> MDPQGDAAQKTDTSHHDQDHPTFNKITPNLAEFAFSLYRQLAHQSNSTNILFSPVSIAAAFAMLSLGAKGDTHDEILEGLNFNLTEIPEAQIHEGFQELLHTLNQPDSQLQLTTGNGLFLSEGLKLVDKFLEDVKKLYHSEAFTVNFGDTEEAKKQINDYVEKGTQGKIVDLVKELDRDTVFALVNYIFFKGKWERPFEVKDTEEEDFHVDQVTTVKVPMMKRLGMFNIQHSKKLSSWVLLMKYLGNATAIFFLPDEGKLQHLENELTHDIITKFLENEDRRSASLHLPKLSITGTYDLKSVLGQLGITKVFSNGADLSGVTEEAPLKLSKAVHKAVLTIDEKGTEAAGAMFLEAIPM;> SIPPEVKFNKPFVFLIIEQNTKAPLFMGRVVNPTQK;> VVGGTEAQRNSWPSQISLQYRSGSSWAHTCGGTLIRQNWVMTAAHCVDRELTFRVVVGEHNLNQNDGTEQYVGVQKIVVHPYWNTDDVAAGYDIALLRLAQSVTLNSYVQLGVLPRAGTILANNSPCYITGWGLTRTNGQLAQTLQQAYLPTVDYAICSSSSYWGSTVKNSMVCAGGDGVRSGCQGDSGGPLHCLVNGQYAVHGVTSFVSRLGCNVTRKPTVFTR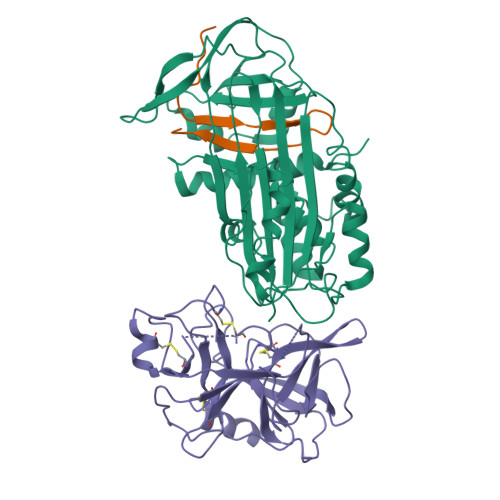VSAYISWINNVIASN>[2x]GHMETNMTFVLKEFDALKSHFNDTVKIILQREKKDKIEDLPNPRKEELQFLTAVLNQLEAKIDELKPRSLASYVHVFYGAMLLVCKDVENNLRVMEKKENS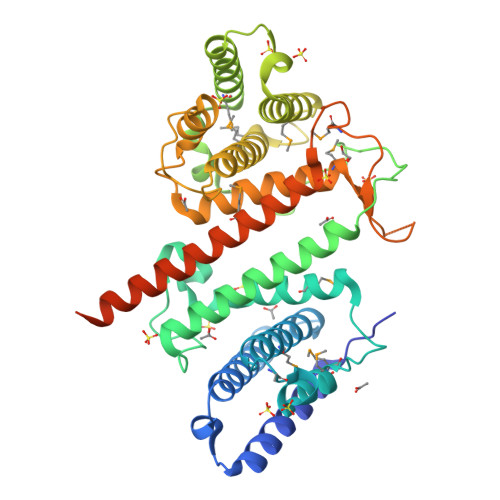LLFTRLMDGMGISDENIPTSEQNIMFYRGLNKFLNFIYESNDSRKGLKKEHFLQVLSLKKIYSLAKLSYEQEEAAENNALAKLTADGKTKANANSFHVEKPIDSSIVEQFKSWDEMKGALHQLILDELSDKNVAKISALSQARSAQLKFLQTMAEQLDKIPNQSLEPSEKMAILAGAMYIVRGQIAQEYGKDPLSNDKISATVIHTGLSTILHANADCCEDKEVLIAAANKFIRHMVIERPEQSNKKITKESVRENNMFSDIAGFQLISVLTLIQNMIKTCRTDAIEACVTKRKEELEALKPKKEGYSIASSVTGYVGSWFKKAPSMSEEGS>MTDFDSLSGTSTTWVNELGSVMTIDVDRKGGVTGYYVNNAPGTGCRGLPYDLSGHAH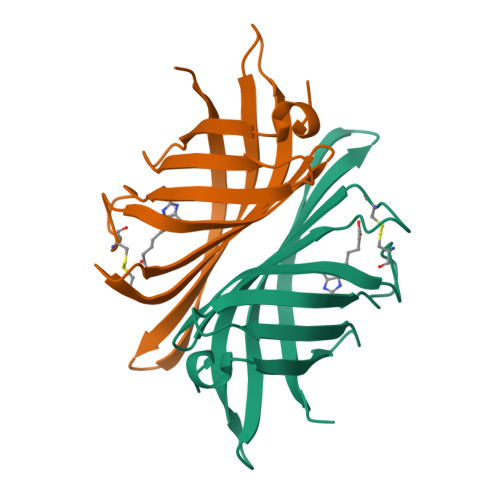GSTIAFSVVWSNGIADCRSATSWAGYARKTFGGGVQIVTQWSLAFVGKAGGKIETGQNVFTYQAATVSESLLTE[20x]>MGHHHH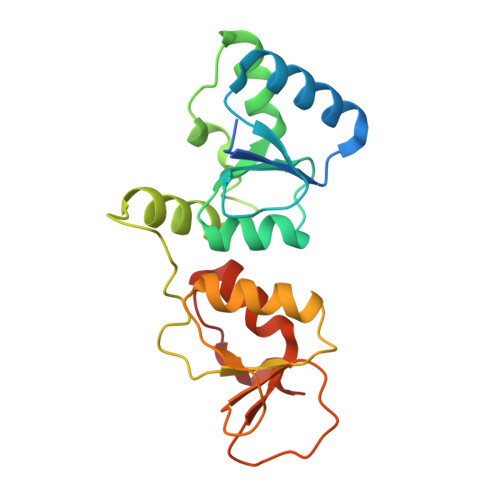HHMKSGRGKKPTRTLVMTSMPSEKQNVVIQVVDKLKGFSIAPDVCETTTHVLSGKPLRTLNVLLGIARGCWVLSYDWVLWSLELGHWISEEPFELSHHFPAAPLCRSECHLSAGPYRGTLFADQPAMFVSPASSPPVAKLCELVHLCGGRVSQVPRQASIVIGPYSGKKKATVKYLSEKWVLDSITQHKVCAPENYLLSQ[3x]> SLGAKPFGEKKFIEIKGRRMAYIDEGTGDPILFQHGNPTSSYLWRNIMPHCAGLGRLIACDLIGMGDSDKLDPSGPERYAYAEHRDYLDALWEALDLGDRVVLVVHDWGSALGFDWARRHRERVQGIAYMEAIAMPIEWADFPEQDRDLFQAFRSQAGEELVLQDNVFVEQVLPGWILRPLSEAEMAAYREPFLAAGEARRPTLSWPRQIPIAGTPADVVAIARDYAGWLSESPIPKLFINAEPGALTTGRMRDFC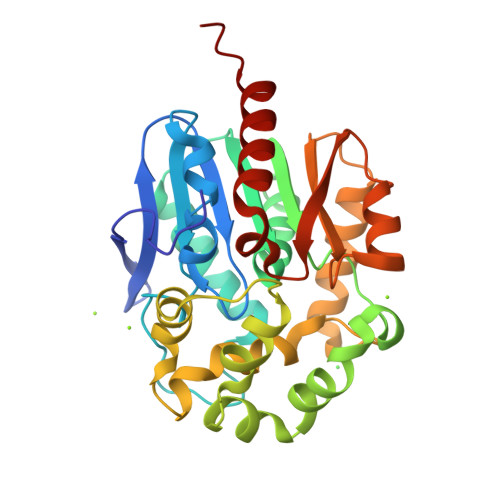RTWPNQTEITVAGAHFIQEDSPDEIGAAIAAFVRRLRPAHH>[8x]GMEPFKQQKVEDFYDIGEELGSGQFAIVKKCREKSTGLEYAAKFIKKRQSRASRRGVSREEIEREVSILRQVLHHNVITLHDVYENRTDVVLILELVSGGELFDFLAQKESLSEEEATSFIKQILDGVNYLHTKKIAHFDLKPENIMLLDKNIPIPHIKLIDFGLAHEIEDGVEFKNIFGTPEFVAPEIVNYEPLGLEADMWSIGVITYILLSGASPFLGDTKQETLAN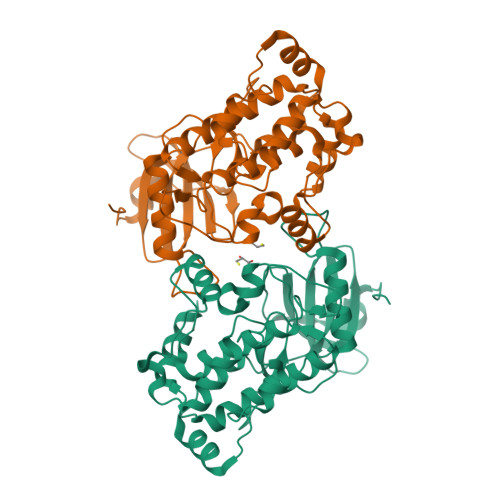ITAVSYDFDEEFFSQTSELAKDFIRKLLVKETRKRLTIQEALRHPWITPVDNQQAMVRRESVVNLENFRKQYVRRRSKLAFSIVSLCNHLTR> GSHMASSCAVQVKLELGHRAQVRKKPTVEGFTHDWMVFVRGPEHSNIQHFVEKVVFHLHESFPRPKRVCKDPPYKVEESGYAGFILPIEVYFKNKEEPRKVRFDYDLFLHLEGHPPVNHLRCEKLTFNNPTE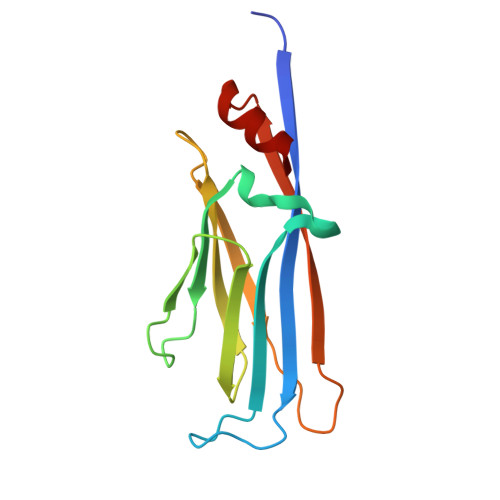DFRRKLLKA>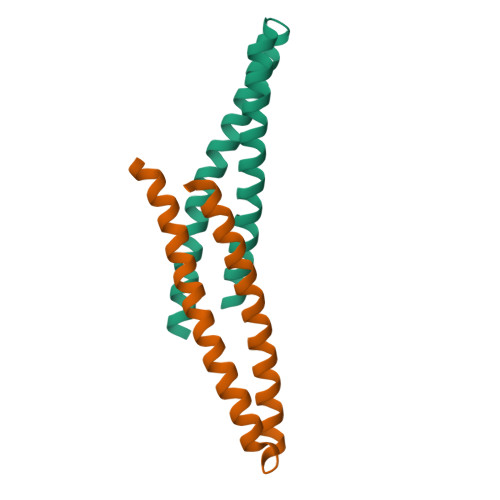GAMEQEAIQRLRDTEEMLSKKQEFLEKKIEQELTAAKKHGTKNKRAALQALKRKKRYEKQLAQIDGTLSTIEFQREALE[4x]2-methyl-4-(2-nitro-4-piperidin-1-yl-phenyl)carbonyl-5-phenyl-1H-pyrazol-3-one | C22 H22 N4 O4 | 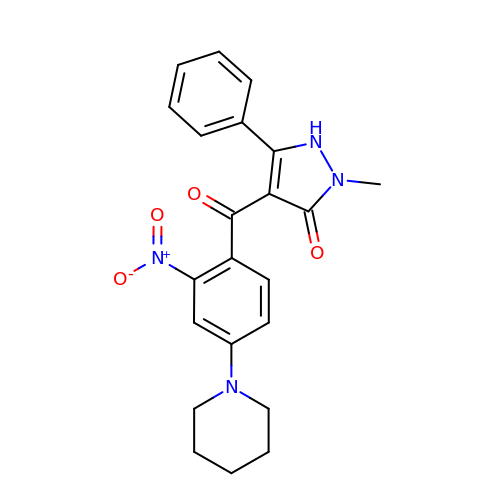LNOSWNGMJQWZSZ-UHFFFAOYSA-N>GPPLPEELVLLERTLADGSTEQIIFSSAGDVNVYDLQALCDKVGWPRRPLTKIAASLRNSYLVATLHSVTMPSKAEGEERKQLIGMARATSDHAFNATIWDVLVDPSYQGQGLGKALMEKVIRTLLQRDISNITLFADNKVVDFYKNLGFEADPQGIKGMFWY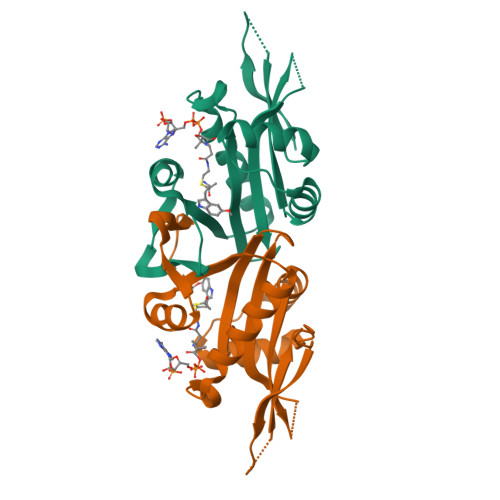PRF[2x]>[2x]MNYPAEPFRIKSVETVSMIPRDERLKKMQEAGYNTFLLNSKDIYIDLLTDSGTNAMSDKQWAGMMMGDEAFAGSENFYHLERTVQELFGFKHIVPTHQGRGAENLLSQLAIKPGQYVAGNMYFTTTRYHQEKNGAVFVDIVRDEAHDAGLNIAFKGDIDLKKLQKLIDEKGAENIAYICLAVTVNLAGGQPVSMANMRAVRELTEAHGIKVFYDATRCVENAYFIKEQE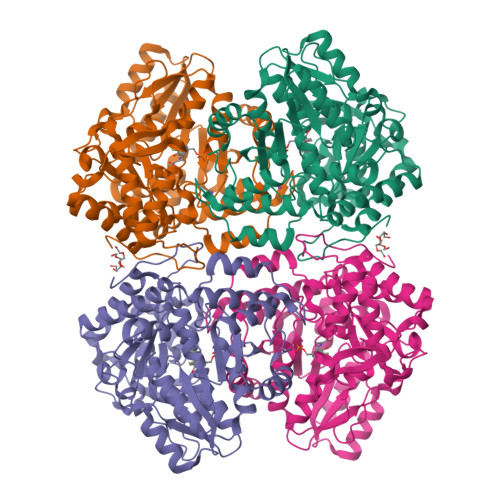QGFENKSIAEIVHEMFSYADGCTMSGKKDCLVNIGGFLCMNDDEMFSSAKELVVVYEGMPSYGGLAGRDMEAMAIGLREAMQYEYIEHRVKQVRYLGDKLKAAGVPIVEPVGGHAVFLDARRFCEHLTQDEFPAQSLAASIYVETGVRSMERGIISAGRNNVTGEHHRPKLETVRLTIPRRVYTYAHMDVVADGIIKLYQHKEDIRGLKFIYEPKQLRFFTARFDYI> ADEFLPTPAPRVTVYVDPPAYPMPRYNYTERWHTTGPIPSPFADGREQPVEVRYATSAAACDMLALIADPQVGRTLWEAVRRHARAYNATVIWYKIESGCARPLYYMEYTECEPRKHFGYCRYRTPPFWDSFLAGFAYPTDDELGLIMAAPARLVEGQYRRALYIDGTVAYTDFMVSLPAGDCWFSKLGAARGYTFGACFPARDYEQKKVLRLTYLTQYYPQEAHKAIVDYWFM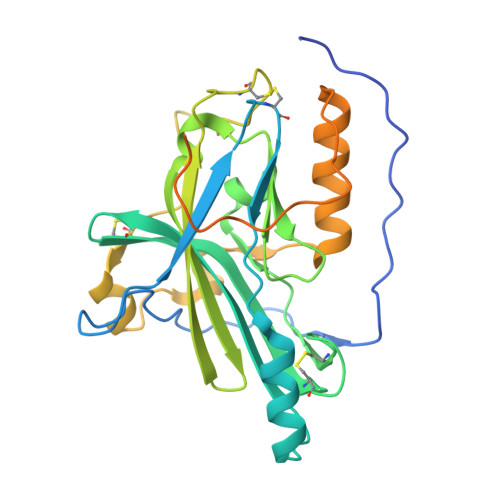RHGGVVPPYFEESKGYEPPPAADGGSPAPPGDDEAREDEGETEDGAAGREGNGGPPGPEGDGESQTPEANGHHHHHH> MLAREAQNIQNPALGAALVWRFCCGYVKTNRVSAPPPLPFLFLVLPIILHQETSEFVKRT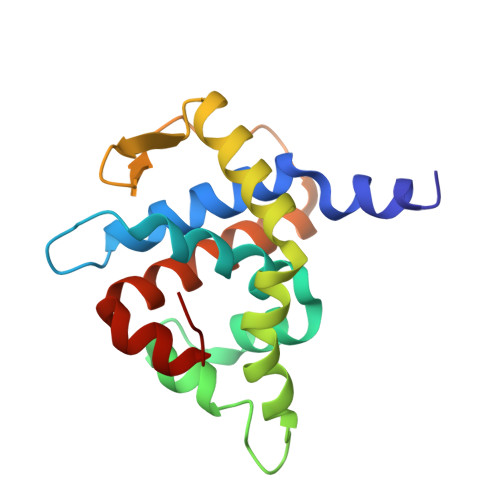YKSSGLRAFAAKFGDSSVSKQDLLFQIHERSIRWRQLSLRSIELAVASDLLKLQDGSDVIPLSKTKARGLSDEVKTLMDLAEKLGSWFGELSIHEVVTTLKVKL In this work, we exhaustively probe the ability of all 36 immobile HJ sequences to form DNA crystals in two different designed systems. Three separate self-assembling DNA crystal systems are described in this report: the “4 × 5” and “4 × 6” designs (collectively referred to as the 4 × N systems), and a third construct with a “scrambled” sequence variant of the 4 × 6 lattices. Self-assembly was mediated by three constituent oligonucleotides: (S1) containing four sequence repeats of either 5 or 6 bases; (S2) composed of 21 bases containing complementary regions to both (S1); and (S3) which forms the second junction crossover. The HJ serves as the fundamental component at the core of each unit, and the ultimate assembly of the full lattice is facilitated by the complementary 2-base sticky ends that tail each duplex.

We hypothesized that it might be possible to introduce other unique immobile sequences that could provide slight perturbations in the junction angle, to potentially reduce the strain in the original system and yield a “relaxed,” periodic lattice. The 4 × 5 system robustly crystallized with 75% of the junctions, and we obtained crystals in all but 9 of 36 sequences. Of the resulting structures, 18 exhibited P32 symmetry with average cell dimensions a = b = 68.85 Å c = 60.09 Å, with only nine retaining the original P3221 symmetry with average cell edges a = b = 68.17 Å c = 60.60 Å. Although the cell parameters between the two symmetries were virtually indistinguishable, the differences between the periodicity of the lattices is dramatic, with vastly different cavity sizes. We hypothesize that even a small difference in junction angles could have a significant global effect on the assembly of the lattice, thereby eliminating the strain in the P3221 lattices. However, in the majority of the crystal structures reported here, the cacodylate anion indeed fits best into the electron density map of our X-ray structures, due to the presence of sodium cacodylate in the crystallization solution.

> GAGCAGACGTGACCGCACTCA;> GGTCA;> TCTGAGTGC;> CGTCTGC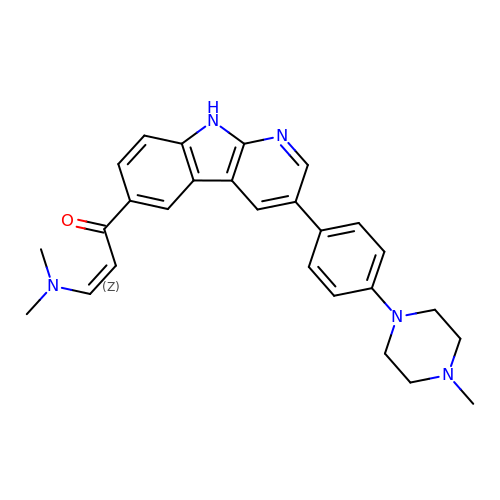3-(dimethylamino)-1-[3-[4-(4-methylpiperazin-1-yl)phenyl]-9~{H}-pyrido[2,3-b]indol-6-yl]prop-2-en-1-one | C27 H29 N5 O | JFOIWAWELQEHHK-KHPPLWFESA-N> MAMDQVNALCEQLVKAVTVMMDPNSTQRYRLEALKFCEEFKEKCPICVPCGLRLAEKTQVAIVRHFGLQILEHVVKFRWNGMSRLEKVYLKNSVMELIANGTLNILEEENHIKDALSRIVVEMIKREWPQHWPDMLIELDTLSKQGETQTELVMFILLRLAEDVVTFQTLPPQRRRDIQQTLTQNMERIFSFLLNTLQENVNKYQQVKTDTSQESKAQANCRVGVAALNTLAGYIDWVSMSHITAENCKLLEILCLLLNEQELQLGAAECLLIAVSRKGKLEDRKPLMVLFGDVAMHYILSAAQTADGGGLVEKHYVFLKRLCQVLCALGNQLCALLGADSDVETPSNFGKYLESFLAFTTHPSQFLRSSTQMTWGALFRHEILSRDPLLLAIIPKYLRASMTNLVKMGFPSKTDSPSCEYSRFDFDSDEDFNAFFNSSRAQQGEVMRLACRLDPKTSFQMAGEWLKYQLSTFLDAGSVNSCSAVGTGEGSLCSVFSPSFVQWEAMTLFLESVITQMFRTLNREEIPVNDGIELLQMVLNFDTKDPLILSCVLTNVSALFPFVTYRPEFLPQVFSKLFSSVTFETVEESKAPRTRAVRNVRRHACSSIIKMCRDYPQLVLPNFDMLYNHVKQLLSNELLLTQMEKCALMEALVLISNQFKNYERQKVFLEELMAPVASIWLSQDMHRVLSDVDAFIAYVGTDQKSCDPGLEDPCGLNRARMSFCVYSILGVVKRTCWPTDLEEAKAGGFVVGYTSSGNPIFRNPCTEQILKLLDNLLALIRTHNTLYAPEMLAKMAEPFTKALDMLDAEKSAILGLPQPLLELNDSPVFKTVLERMQRFFSTLYENCFHILGKAGPSMQQDFYTVEDLATQLLSSAFVNLNNIPDYR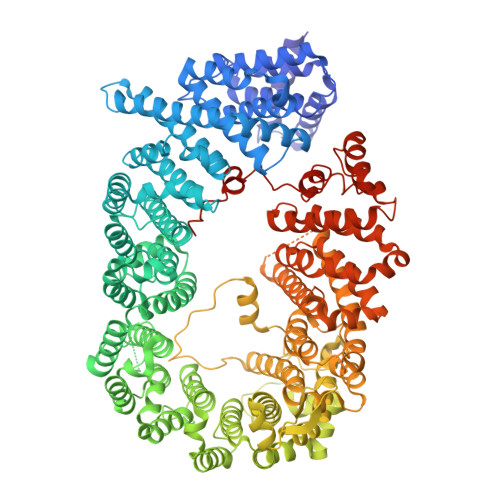LRPMLRVFVKPLVLFCPPEHYEALVSPILGPLFTYLHMRLSQKWQVINQRSLLCGEDEAADENPESQEMLEEQLVRMLTREVMDLITVCCVSKKGADHSSAPPADGDDEEMMATEVTPSAMAELTDLGKCLMKHEDVCTALLITAFNSLAWKDTLSCQRTTSQLCWPLLKQVLSGTLLADAVTWLFTSVLKGLQMHGQHDGCMASLVHLAFQIYEALRPRYLEIRAVMEQIPEIQKDSLDQFDCKLLNPSLQKVADKRRKDQFKRLIAGCIGKPLGEQFRKEVHIKNLPSLFKKTKPMLETEVLDNDGGGLATIFEP> MEYTPWLIAGLGNPGNKYYGTRHNVGFEMVDRIAAEEGITMNTNQFKSLLGTGSIGEVPVLVVKPQSYMNYSGEAIGPLAAYYQVPLRHILLIYDDTSLPNGVLRLQKKGGHGRHNGLQNVIEHLDGRREFPRLSIGIGSPPGKMDPRAFLLQKFSSEERVQIDTALEQGVDAVRTLVLKGFSGSTERFNLV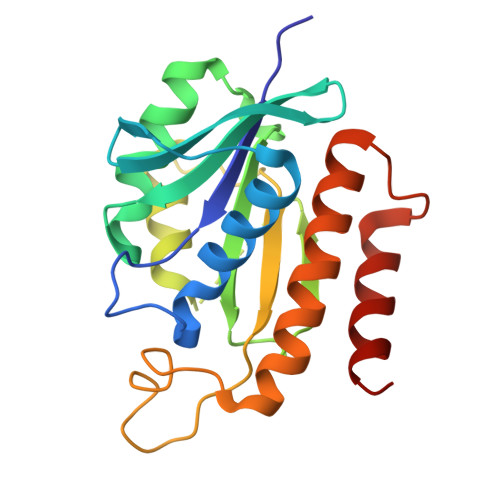QKLEHHHHHH>[2x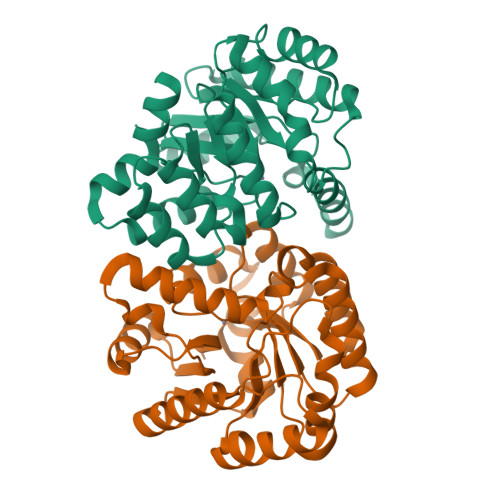]MSLIIDGHTHVILPVEKHIKIMDEAGVDKTILFSTSIHPETAVNLRDVKKEMKKLNDVVNGKTNSMIDVRRNSIKELTNVIQAYPSRYVGFGNVPVGLSENDTNSYIEENIVNNKLVGIGELTPASGQIKSLKPIFKYSMDSGSLPIWIHAFNPLVLQDIKEIAELCKAFPKVPVILGHMGGSNWMTAVELAKEIQNLYLDTSAYFSTFVLKIVINELPLKCIFGTDMPFGDLQLSIEAIKKMSNDSYVANAVLGDNISRLLNIEGHHHHHH>MGSSHHHHHHENLYFQSNAETVAAIKTLIQQLAQSTDQFGRAEINDALRELQYSLETPFDTVMRMSLDTAQVAVARIGSDLGLFKHLSQCASPQSAEELADHLGCGRELMSRLLRYMASVRMVQQTDDIKYISSNITQTLAVPGLEAGMRHAFENLWPVLMALPDFLAERKYPDIVDAKDTAFQKAFNTDQDCFHWLATQPTRIANFKVLLTDERTPNFLSTFPLEKELGSWSAEPEKALFVDIGGGMGHACIRLREKYPNQPGRVILQDLPPVLQAAQATLPLSGIESMPHNFHTPQPVQGAKFYFLRLILRDFPDHQALEILQN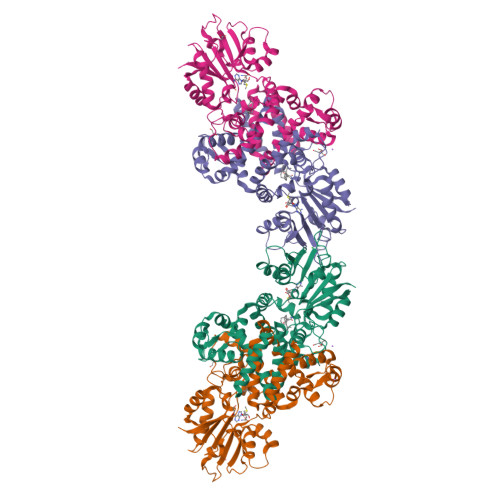IVPAMDAESRIVIDDGVPPEKGARWAETGTDICIMSALGSKERTQRQWEELAAKAGLQLQALYQYTWPVVNAAMVFSLQ[2x]> MSLKVQGYANVVTLPNVTGRVIIVGDIHGCRAQLEDLLRAVSFKQGSDTLVAVGDLVNKGPDSFGVVRLLKRLGAYSVLGNHDAKLLKLV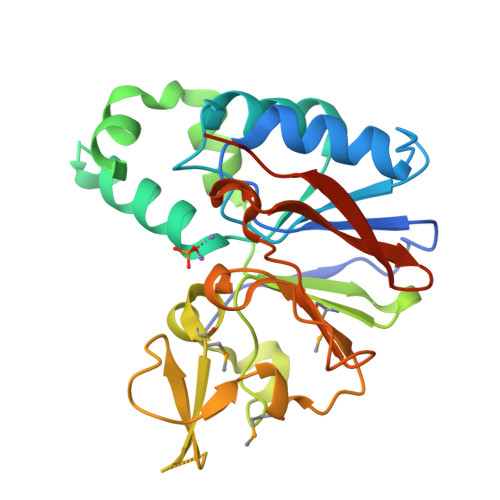KKLGKKECLKGRDAKSSLAPLAQSIPTDVETYLSQLPHIIRIPAHNVMVAHAGLHPQRPVDRQYEDEVTTMRNLIEKEQEATGGVTLTATEETNDGGKPWASMWRGPETVVFGHDARRGLQEQYKPLAIGLDSRCVYGGRLSAAVFPGGCIISVPGWNGASAAAEGHHHHHH>[4x]MMPTEYPATAEESVDVITDALLTASRLLVAISAHSIAQVDENITIPQFRTL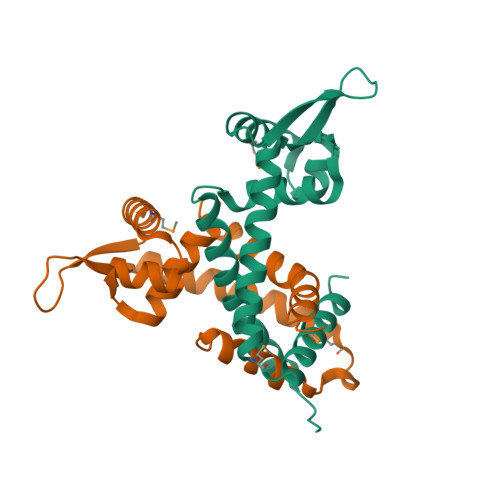VILSNHGPINLATLATLLGVQPSATGRMVDRLVGAELIDRLPHPTSRRELLAALTKRGRDVVRQVTEHRRTEIARIVEQMAPAERHGLVRALTAFTEAGGEPDARYEIERSHHHHHH>[2x]QSITDYNYKKPLHNDYQILDKSKIFGSNSGSFVMYSMAADAYYIYNEKESRKRYSPNS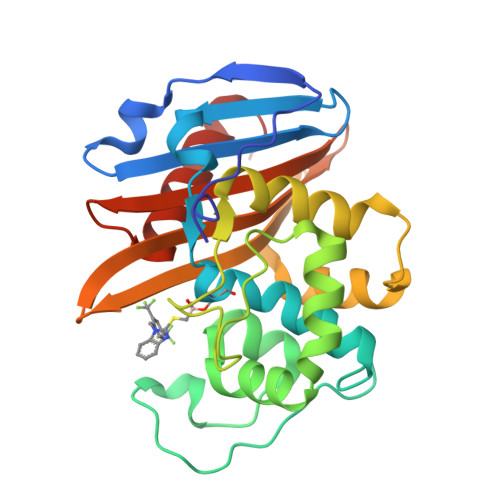TYKIYLAMFGLDRHIINDENSRMSWNHKHYPFDAWNKEQDLNTAMQNSVNWYFERISDQIPKNYTATQLKQLNYGNKNLGSYKSYWMEDSLKISNLEQVIVFKNMMEQNNHFSKKAKNQLSSSLLIKKNEKYELYGKTGTGIVNGKYNNGWFVGYVITNHDKYYFATHLSDGKPSGKNAELISEKILKEMGVLNGQ In this process, small GTPase Rab5 functions as a master regulator of the early endosomal biogenesis. Rabex-5 is a specific GEF for Rab5, Rab17, and Rab21. Rabaptin-5 is a key effector of Rab5 and plays an important role in both homotypic and heterotypic fusions of early endosomes. The GEF activity of Rabex-5 is autoinhibited by its CC domain and is activated by the binding of Rabaptin-5 via its C2-1 domain.

The asymmetric unit contains two Rab5-Rabex-5Δ-Rabaptin-5C212 complexes related by a twofold non-crystallographic symmetry. However, in the R3Δ complex, Rabaptin-5C212 adopts a linear conformation and the Rabex-5 GEF domain is displaced with a completely exposed substrate-binding site. Indeed, in the structure of the R3Δ complex, although Rabex-5CC still forms a tight three-helix bundle with the C-terminal regions of Rabaptin-5C212, Rabaptin-5C212 forms a linear two-helix bundle which is different from the V-shaped conformation but similar to that in the Rabex-5CC-Rabaptin-5C212 complex and the GAT-Rabaptin-5C212 complex. The GEF domain is dislodged from the three-helix bundle and interacts with the N-terminal regions of Rabaptin-5C212, and the substrate-binding site is completely exposed to bind Rab5. The GEF domain of Rabex-5 interacts via a small portion of the opposite side of the substrate-binding site with a small portion of the N-terminal regions of Rabaptin-5C212. The overall structure of the nucleotide-free Rab5 differs from the nucleotide-bound Rab5 in the conformations of the P-loop and the switch regions. Nevertheless, the interactions between Rabex-5 and Rab5 are similar to those between Rabex-5 and Rab21, suggesting that Rabex-5 may activate Rab5 via a similar mechanism as for Rab21. Moreover, in the R3Δ structure, Rabaptin-5C212 also assumes a linear conformation but two Rabaptin-5C212 dimerize through the middle regions (residues 590–600) between the GAT-binding site and the Rabex-5CC-binding site. The binding of the GDP-bound Rab5 to Rabex-5 induces further conformational changes of the Rabex-5-Rabaptin-5 complex such that Rabaptin-5C212 transforms from the V-shaped to the linear conformation, the GEF domain is dislodged from Rabex-5CC and the C-terminal regions of Rabaptin-5C212, and the substrate-binding site is completely exposed to the solvent to bind Rab5 as observed in the R3Δ structure (State III). Similarly, the theoretical scattering curve calculated from the R3Δ model fits well with the experimental SAXS data for both R3 and R3Δ complexes (goodness of fit χ = 0.68 and 0.96, respectively), and the theoretical P(r) distribution of the R3Δ model is also in good agreement with the experimental P(r) distributions of both R3 and R3Δ complexes. These results indicate that the R3 and R3Δ complexes assume mainly the linear conformation as observed in the R3Δ structure in solution.

>MGHHHHHHSIETDRVSKEFIEFLKTFHKTGQEIYKQTKLFLEGMHYKRDLSIEEQSECAQDFYHNVAERMQTRGKVPPERVEKIMDQIEKYIMTRLYKYVFCPETTDDEKKDLAIQKRIRALRWVTPQMLCVPVNEDIPEVSDMVVKAITDIIEMDSKRVPRDKLACITKCSKHIFNAIKITKNEPASADDFLPTLIYIVLKGNPPRLQSNIQYITRFCNPSRLMTGEDGYYFTNLCCAVAFIEKLDAQSLNLSQEDFDRYMSGQTSPRKQMYKNLDLLSQLNERQERIMNEAKKLEKDLIDWTDGIAREVQDIVEK[2x];>[2x]SGNKICQFKLVLLGESAVGKSSLVLRFVKGQFHEFQESTIGAAFLTQTVCLDDTTVKFEIWDTAGQERYHSLAPMYYRGAQAAIVVYDITNEESFARAKNWVKELQRQASPNIVIALSGNKADLANKRAVDFQEAQSYADDNSLLFMETSAKTSMNVNEIFMAIAKKLPKN;>METRDQVKKLQLMLRQANDQLEKTMKDKQELEDFIKQSSEDSSHQISALVLRAQASEILLEELQQGLSQAKRDVQEQMAVLMQSREQVSEEL[4x]> TQPLSKTWELSLYELQRTPQEAITDGLEIVVSPRSLHSELMCPICLDMLKNTMTTKECLHRFCADCIITALRSGNKECPTCRKKLVSKRSLRPDPNFDALISKIYPSMHRTTRIKITELNPHLMCVLCGGYFIDATT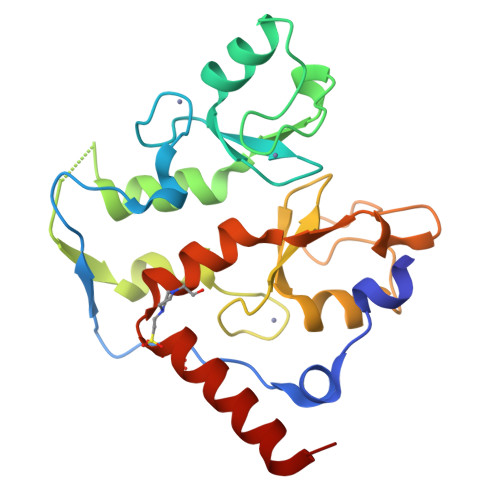IIECLHSFCKTCIVRYLETSKYCPICDVQVHKTRPLLNIRSDKTLQDIVYKLVPGLFKNEMKRRRDFYAAHPSA> VDCSEYPKPACTNEYRPLCGSDNKTYGNKCNFCNAVVESNGTLTLSH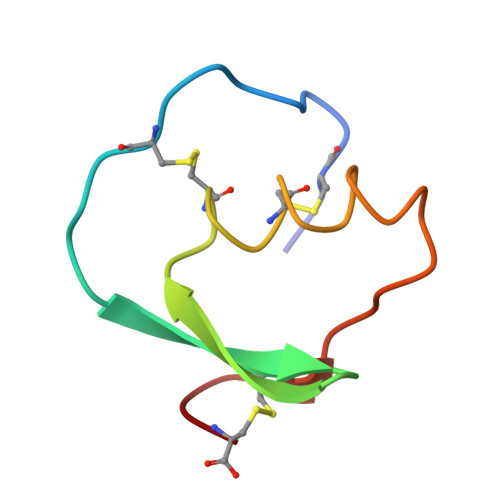FGKC>AELPTHYGTIIKTLRKYMKLTQSKLSERTGFSQNTISNHENGNRNIGVNEIEIYGKGLGIPSYILHRISDEFKEKGYSPTLNDFGKFDKMYSYVNKAYYNDGDIYYSSYDLY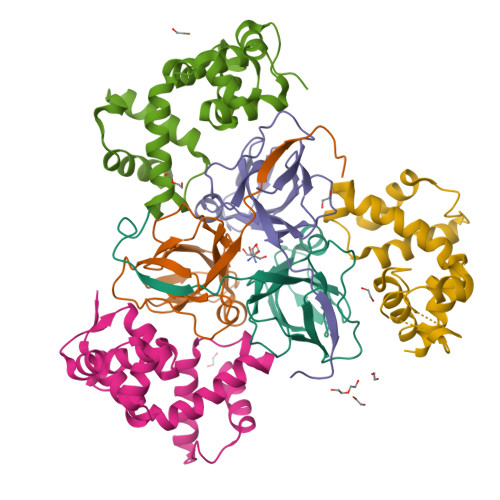DETIKLLELLKESKINVNDIDYDYVLKLYKQILST[6x];>[6x]MSTTLAIVRLDPGLPLPSRAHDGDAGVDLYSAEDVELAPGRRALVRTGVAVAVPFGMVGLVHPRSGLATRVGLSIVNSPGTIDAGYRGEIKVALINLDPAAPIVVHRGDRIAQLLVQRVELVELVEVSSFDEAGLA>MELIRIAMKKDLENDNSLMNKWATVAGLKNPNPLYDFLNHDGKTFNEFSSIVNIVKSQYPDREYELMKDYCLNLDVKTKAARSALEYADANMFFEIEDVLIDSMISCSNMKSKEYGKVYKIHRELSNSVITEFEAVKRLGKLNIKTPEMNSFSRLLLLYHYLSTGNFSPMAQLIKQIDLSEISENMYIRNTYQTRVHVLMSNIKLNENSLEECREYSKKALESTNILRFQVFSYLTIGNSLLFSNYELAQENFLKGLSISVQNENYNMIFQQALCFLNNVWRKENKWINFESDSIMDLQEQAHCFINFNENSKAKEVLDKLDLLVHNDNELAMHYYLKGRLEQNKACFYSSIEYFKKSNDKFLIRLPLLELQKMGENQKLLELLLLLEYA[2x];>GMPRGA[2x]

The arbitrium system comprises three phage genes: (1) AimP, encoding the peptide that is processed into a 6 aa signaling peptide extracellularly, (2) AimR, encoding the intracellular receptor of AimP that is predicted to be structurally similar to RRNPP regulators, and (3) AimX, encoding a putative long non-coding DNA that functions as the negative regulator of lysogeny. As a transcription factor, AimR dimer induces expression of AimX, which promotes lytic cycle. The concentration of AimP will eventually reach the point that its uptake by newly infected bacteria will be high enough to bind AimR and abolish transcriptional activation of AimX, thereby shifting the phage into lysogenic cycle. As predicted from its similarity with RRNPP proteins, the structure of AimR is characterized by two domains, i.e., the N-terminal HTH DNA-binding domain (residues 1–73) and the C-terminal TPR domain (residues 79–386), which are connected by a short linker (residues 74–78).

The electron density of the N-terminus of AimR within the AimR-AimP complex was of better quality; using the structure of apo AimR as a model, the binary complex AimR-AimP was solved by molecular replacement and refined to 2.00 Å resolution. In the structure of AimR-AimP complex, two molecules of AimR are present in the asymmetric cell unit. One molecule of the AimP hexapeptide (GMPRGA) binds to one molecule AimR. The TPR domain of AimR forms a deep concave pocket that accommodates a molecule of AimP, with a buried interface area of 758.6 Å2. The C-terminus alanine of AimP is facing the interior of the pocket, whereas the N-terminal glycine is located at the entry point. In vitro ITC assay demonstrates that full-length AimR specifically binds AimP with a Kd of 40 nmol/L. The interaction between AimR and AimP includes an extensive network of hydrogen bonds and hydrophobic contacts. The oxygen atoms from the peptide backbone of AimR form hydrogen bonds with four AimP residues: Q299AimR and E300AimR interact with the nitrogen moiety of G1AimP, N239AimR forms hydrogen bonds with P3AimP, N202AimR interacts with G5AimP, and R228AimR contacts the oxygen moieties of A6AimP, whereas five hydrophobic residues from AimR (L205, L242, F276, F362 and L363) are involved in van der Waals interactions with the side chain of M2AimP. As opposed to the classical interaction between RRNPP and the signaling peptide in bacteria that does not include side chain-specific contacts, the guanidinium group of R4AimP forms hydrogen bonds with three residues in AimR, namely N206, N329 and D360. However, our structure indicates that in the spBeta-derived AimR-AimP complex AimRs still exist as a dimer.> MGAQVSSQKVGAHENSNRAYGGSTINYTTINYYKDSASNAASKQDYSQDPSKFTEPLKDVLIKTAPALNSPNVEACGYSDRVLQLTIGNSTITTQEAANSVVAYGRWPEFIRDDEANPVDQPTEPD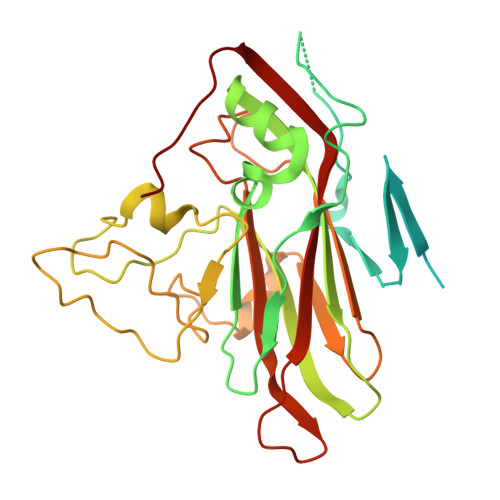VATCRFYTLDTVMWGKESKGWWWKLPDALRDMGLFGQNMYYHYLGRSGYTVHVQCNASKFHQGALGVFAIPEYCLAGDSDKQRYTSYANANPGEKGGKFYSQFNRDTAVTSPKREFCPVDYLLGCGVLLGNAFVYPHQIINLRTNNSATIVLPYVNAMAIDSMVKHNNWGIAILPLSPLDFAQESSVEIPITVTIAPMCSEFNGLRNVTAPKFQ>ADCAKGKIEFSKYNEDDTFTVKVDGKEYWTSRWNLQPLLLSAQLTGMTVTIKSSTCESGSGFAEVQFNND[1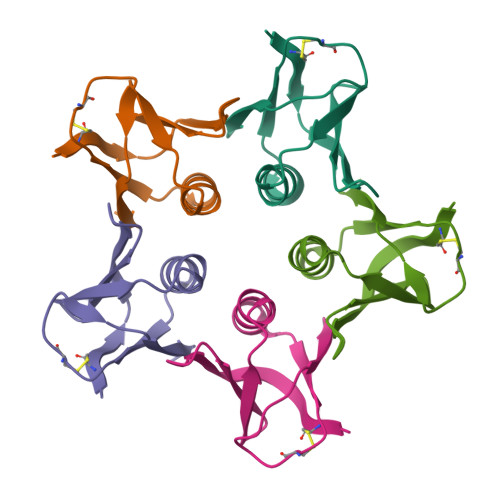0x]(4-oxo-5-phenyl-3,4-dihydrothieno[2,3-d]pyrimidin-2-yl)methyl 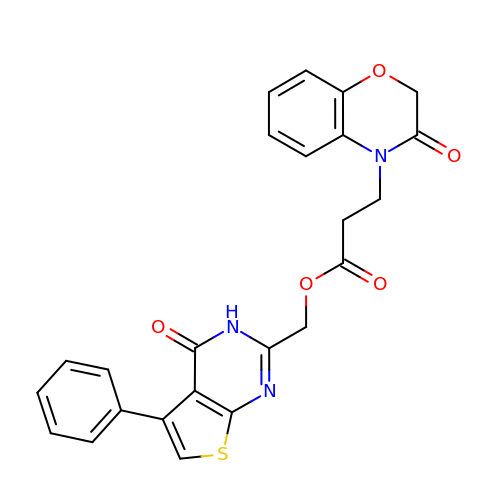3-(3-oxo-2,3-dihydro-4H-1,4-benzoxazin-4-yl)propanoate | C24 H19 N3 O5 S | YOFCRYWWKQMPEW-UHFFFAOYSA-N> GPEIVDTCSLASPASVCRTKHLHLRCSVDFTRRTLTGTAALTVQSQEDNLRSLVLDTKDLTIEKVVINGQEVKYALGERQSYK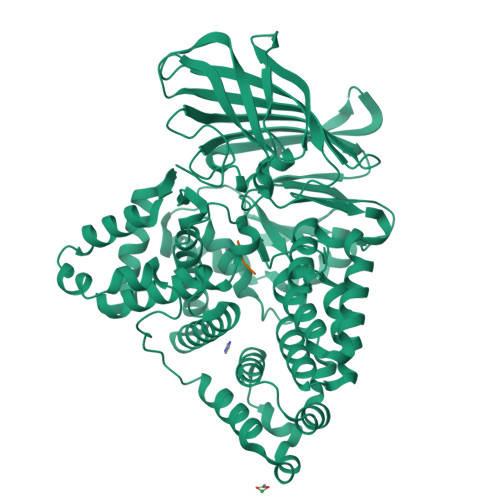GSPMEISLPIALSKNQEIVIEISFETSPKSSALQWLTPEQTSGKEHPYLFSQCQAIHCRAILPCQDTPSVKLTYTAEVSVPKELVALMSAIRDGETPDPEDPSRKIYKFIQKVPIPCYLIALVVGALESRQIGPRTLVWSEKEQVEKSAYEFSETESMLKIAEDLGGPYVWGQYDLLVLPPSFPYGGMENPCLTFVTPTLLAGDKSLSNVIAHQISHSWTGNLVTNKTWDHFWLNEGHTVYLERHICGRLFGEKFRHFNALGGWGELQNSVKTFGETHPFTKLVVDLTDIDPDVAYSSVPYEKGFALLFYLEQLLGGPEIFLGFLKAYVEKFSYKSITTDDWKDFLYSYFKDKVDVLNQVDWNAWLYSPGLPPIKPNYDMTLTNACIALSQRWITAKEDDLNSFNATDLKDLSSHQLNEFLAQTLQRAPLPLGHIKRMQEVYNFNAINNSEIRFRWLRLCIQSKWEDAIPLALKMATEQGRMKFTRPLFKDLAAFDKSHDQAVRTYQEHKASMHPVTAMLVGKDLKVD;> PGP>MSASIRDAGVADLPGILAIYNDAVGNTTAIWNETPVDLANRQAWFDTRARQGYPILVASDAAGEVLGYASYGDWRPFEGFRGTVEHSVYVRDDQRGKGLGV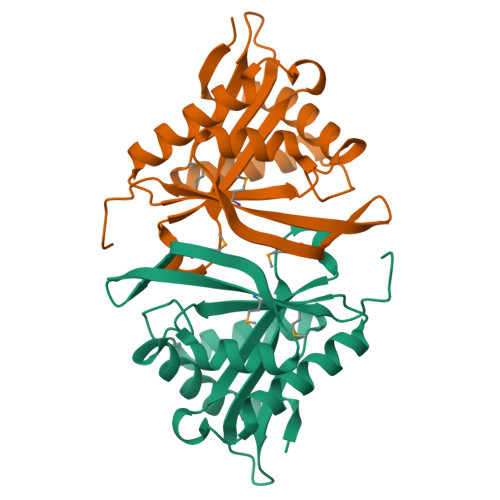QLLQALIERARAQGLHVMVAAIESGNAASIGLHRRLGFEISGQMPQVGQKFGRWLDLTFMQLNLDPTRSAP[2x]> GSMGLLTILKKMKQKERELRLLMLGLDNAGKTTILKKFNGEDVDTISPTLGFNIKTLEHRGFKL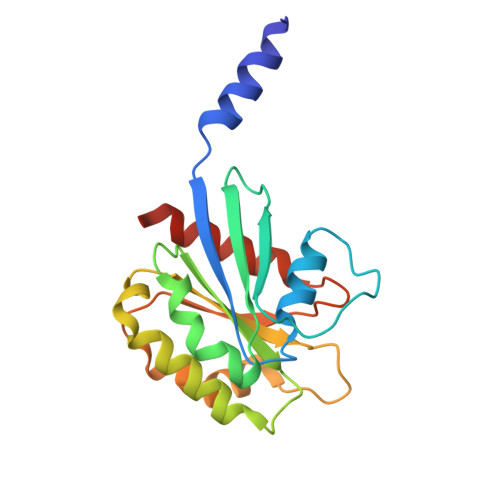NIWDVGGQKSLRSYWRNYFESTDGLIWVVDSADRQRMQDCQRELQSLLVEERLAGATLLIFANKQDLPGALSCNAIQEALELDSIRSHHWRIQGCSAVTGEDLLPGIDWLLDDISSRVFTAD> SGQRWELALGRFWDYL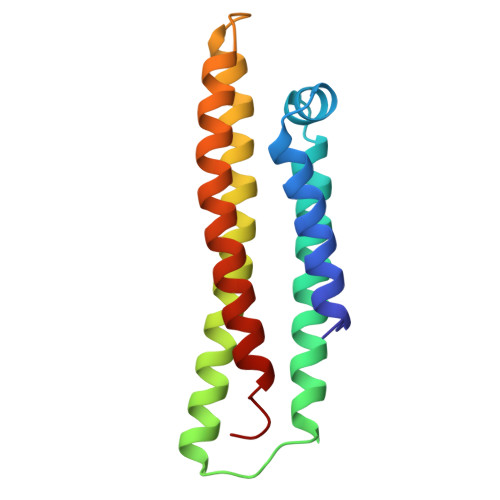RWVQTLSEQVQEELLSSQVTQELRALMDETMKELKAYKSELEEQLTPVAEETRARLSKELQAAQARLGADMEDVCGRLVQYRGEVQAMLGQSTEELRVRLASHLRKLRKRLLRDADDLQKRLAVYQAG> MNYKLTLHPGSNPVEEFTSIPHGVTSLDLSLNNLYSISTVELIQAFANTPASVTSLNLSGNSLGFKNSDELVQILAAIPANVTSLNLSGNFLSYKSSDELVKTLAAIPFTITVLDLGWNDFSSKSSSEFKQAFSNLPASITSLNLR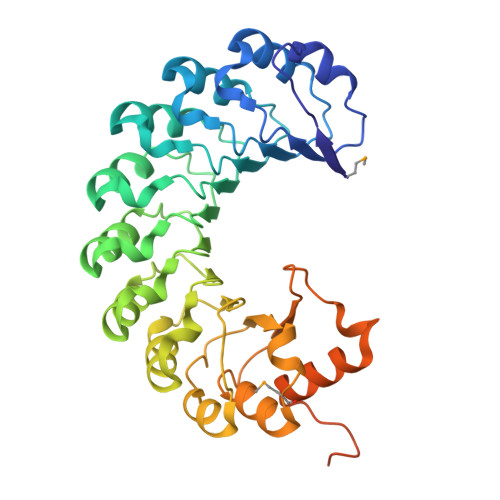GNDLGIKSSDELIQILAAIPANVNSLNLRGNNLASKNCAELAKFLASIPASVTSLDLSANLLGLKSYAELAYIFSSIPNHVVSLNLCLNCLHGPSLENLKLLKDSLKHLQTVYLDYDIVKNMSKEQCKALGAAFPNIQKIILVDKNGKEIHPSHSIPISNLIRELSGKADVPSLLNQCLIFAQKHQTNIEDLNIPDELRESIQTCKPLLEHHHHHH>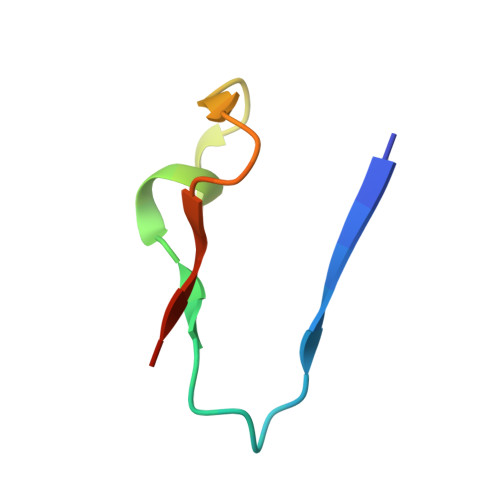 SFALGLRKDCRAEIVEKFTEPGTVIRINEVVAALKA> GSEAAGGEQRELLIQRLRAAVHYTTGCLCQDVAEDKGVLFSKQTV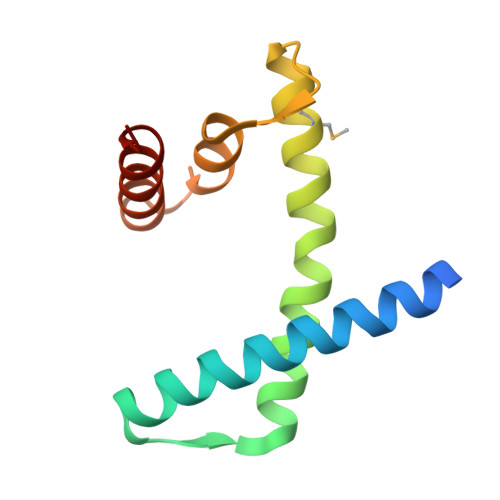AAISEITFRQCENFARDLEMFARHAKRSTITSEDVKLLARRSNSLLKYITQKSDELASSNME>VRLPGLAAMRQGTRLFTPEQGEDLREALRRRRGSFQTTCEVTSETTFAAARRLREKASALAALNFASAKNPGGGFLGGAQAQEEDLCRGSGLYFSLTSPQAEPYYAVNRQSHSALYTDHLIYSPQVPIFRDDAGQLLPAPVPVNIITAPAPNAGAVAQSRPEQLPQVLPTLRERARRVLGVAAWMEQTHLVLGAWGCGVFRNDPAGVARTFRELLEGEAQGAFEHVTFAVLDNHPQHPTLGAFRRELESLCLP[6x]

Despite the abundance of PARP1, most of the PAR generated by DNA damage is rapidly degraded, with a half-life of less than 1 min by poly (ADP-ribose) glycohydrolase (PARG). The radio-resistant bacterium D. radiodurans encodes a PARG homolog, DrPARG, whose expression is upregulated after radiation damage, so it might play an important role in DNA repair. Our study demonstrates that DrPARG is involved in catalyzing the breakdown of endogenous PAR and DNA repair in D. radiodurans. From observing the structural peculiarities of DrPARG, we show that although previously thought to be an obligate exo-glycohydrolase, bacterial PARG could exert both exo- and endo-glycohydrolase functions.

Therefore, we attempted to obtain crystals of DrPARG in complex with ADP-ribose. Crystals were found in several similar conditions, but they belonged to different space groups. Notably, the 28 N-terminal residues of these solved structures from different space groups, including P21, P32, P3221, and P212121, were not well defined in the electron density maps, which suggests that this phenomenon did not result from crystal packing. In fact, the missing residues located in the intrinsically disordered N-terminal region of DrPARG and might be highly flexible. The structural flexibility may reflect the multiple space groups observed in X-ray crystallography because packing patterns are constantly influenced by the flexible regions during crystallization.To gain further insight into the structural conversions in pore formation, we chose pleurotolysin (Ply), a MACPF protein consisting of two components, PlyA and PlyB, from Pleurotus ostreatus. Previous studies have shown that PlyA binds membranes and is required to recruit the pore-forming MACPF protein PlyB to the membrane surface. PlyA and PlyB together form relatively small and regular pores in liposomes. The membrane attack complex/perforin-like family (MACPF) proteins form the largest superfamily of pore-forming proteins identified to date.

To further probe TMH2 function, a third PlyB disulphide lock was created to join strands β4 of the central β-sheet to β5 of TMH2, PlyBV277C,K291C (TMH2 strand lock). Cryo-EM and modelling analysis showed that the central β-sheet was open to the same extent as in the TMH1 lock (49° ± 8°). This result provides an interesting contrast to the consequences of the TMH2 helix lock and highlights that simply restricting TMH2 movement through locking strands β4 and β5 does not prevent opening of the core sheet. The restrictions enforced by the TMH2 strand lock are, however, sufficient to prevent extension of the TMH2 hairpin since no density is seen extending into the membrane. These data collectively imply that neither TMH region can enter the membrane without the other, suggesting that the TMH sequences have evolved for cooperative folding and assembly.

>[2x]AYAQWVIIIIHNVGSKDVKIKNLKPSWGKLHADGDKDTEVSASKYEGTVIKPDEKLQINACGRSDAAEGTTGTFDLVDPADGDKQVRHFYWDCPWGSKTNTWTVSGSNTKWMIEYSGQNLDSGALGTITVDTLKK;> SQAGDTLNDVIQDPTRRNKLINDNNLLKGIIMGRDGPVPSSRELIVRPDTLRAIINNRATIETTTMKSMYTSSRYLFPQGRIDFTTPDSGFDDVIKLSPQFTSGVQAALAKATGTEKREALQNLFQEYGHVFRTKVHIGGVLSAHTMETFSKLNVKYIVNGGDYTKIQNTEEWVASTNQSEHWRVIEVTEVTAVADLLPQPIRGQVKDLLKPLLGKWVDVEKVPGLESLPVSVYRPKGAIPAGWFWLGDTADASKALLVKPTLPARSGRNPALTSLHQGSGMTEQPFVDLPQYQYLSTYFGSFAHDTPPGSTLRGLRPDHVLPGRYEMHGDTISTAVYVTRPVDVPFPEDECFDLKSLVRVKLPGSGNPPKPRSALKKSMVLFDSGEK A plant called Arabidopsis thaliana has a light-sensitive protein called ZEITLUPE (or ZTL for short) that helps it keep its circadian clock in sync with the cycle of night and day. In Arabidopsis thaliana, three LOV domain containing proteins ZTL, FLAVIN-BINDING, KELCH REPEAT, F-BOX 1 (FKF1), and LOV KELCH PROTEIN 2 (LKP2) act in circadian timing and seasonal flowering. Recent research indicates that their divergent roles in the circadian clock and photoperiodic flowering may enable interrogation of how chemistry regulates PAS/LOV protein function to select for signaling pathways. These proteins retain analogous elements, where an N-terminal LOV domain regulates activity of a C-terminal E3 ubiquitin ligase to target clock proteins for degradation in a time dependent manner. LOV domains are typified by blue-light induced formation of a C4a adduct between a conserved Cys residue and a bound flavin (FAD, FMN or riboflavin) cofactor.

Dark and light state structures of V48I:G80R confirm concerted movement of Q154 that is linked to conformational changes in V/I48. Light state crystals of V48I:G80R were obtained as follows. Prior to setting screens V48I:G80R protein was exposed to a broad spectrum white flood light (150 W), while on ice for two minutes. Comparing the dark-state to V48I:G80R grown in the light, confirms density for the C4A adduct and confirms direct crystallization of the light-state. For light-state structures clear density is observed for the adduct state in two of four molecules. Difference density maps of the light-state molecule indicate that adduct formation is coupled to rotation of Q154 to a buried position. Unexpectedly, rotation of Q154 requires concerted movement of I48 that reorients the Ncap. In the light, V48I disrupts rotation of Q154 to the buried conformation, thereby leading to a predominantly exposed conformation regardless of lighting conditions. Further, the light-state V48I:G80R molecule indicates partial Q154 rotation to a buried conformation that is impeded by V48I. This impediment does not allow robust sampling of the buried conformation under any lighting conditions and coincides with constitutively high TOC1/PRR5 degradation in V48I containing variants.

>[4x]GGPIPYPVGNLLHTAPCGFIVTDAVEPDQPIIYVNTVFEMVTGYRAEEVLGRNCRFLQCRGPFAKRRHPLVDSMVVSEIRKCIDEGIEFQGELLNFRKDGSPLMNRLRLTPIYGDDDTITHIIGIQFFIETDIDLGP4-[4-[5-[(2~{S},3~{R},4~{R},5~{S},6~{R})-6-(hydroxymethyl)-3,4,5-tris(oxidanyl)oxan-2-yl]-4~{H}-1,2,4-triazol-3-yl]phenyl]benzoic acid 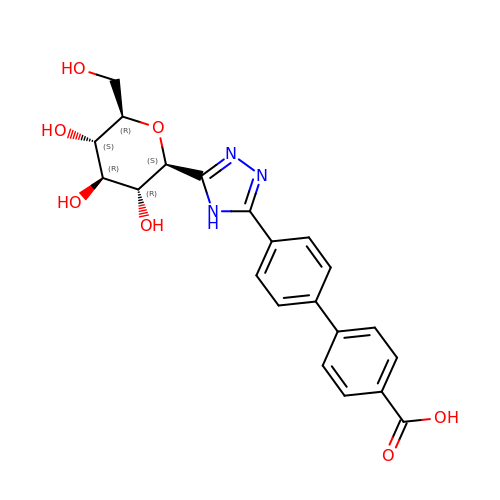| C21 H21 N3 O7 | UQZVJUDMJCTDEV-UYTYNIKBSA-N1,1'-[[1,1'-biphenyl]-4,4'-diylbis(methylene)]bis{4-[(4-chlorophenyl)(methyl)amino]quinolin-1-ium} | 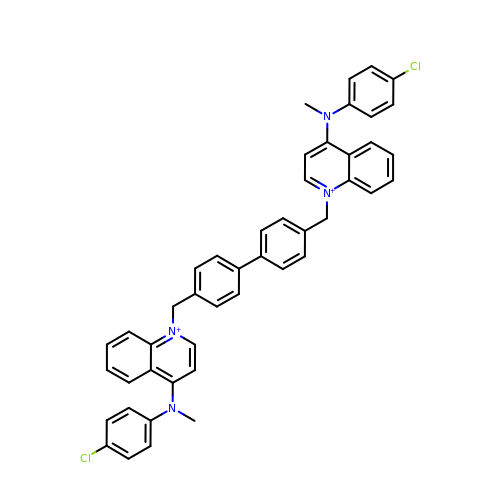C46 H38 Cl2 N4 | QGYGTMZEJNOHNU-UHFFFAOYSA-N>[2x]SMSSWKKQAEDIKKIFEFKETLGTGAFSEVVLAEEKATGKLFAVKCIPKKALKGKESSIENEIAVLRKIKHENIVALEDIYESPNHLYLVMQLVSGGELFDRIVEKGFYTEKDASTLIRQVLDAVYYLHRMGIVHRDLKPENLLYYSQDEESKIMISDFGLSKMEGKGDVMSTACGTPGYVAPE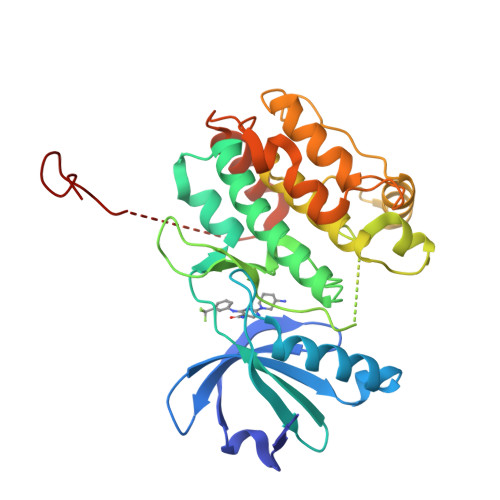VLAQKPYSKAVDCWSIGVIAYILLCGYPPFYDENDSKLFEQILKAEYEFDSPYWDDISDSAKDFIRNLMEKDPNKRYTCEQAARHPWIAGDTALNKNIHESVSAQIRKNFAKSKWRQAFNATAVVRHMRKLHLGSSLD>[3x]SGFVCNTCPEKWINFQRKCYYFGKGTKQWVHARYACDDMEGQLVSIHSPEEQDFLTKHASHTGSWIGLRNLDLKGEFIWV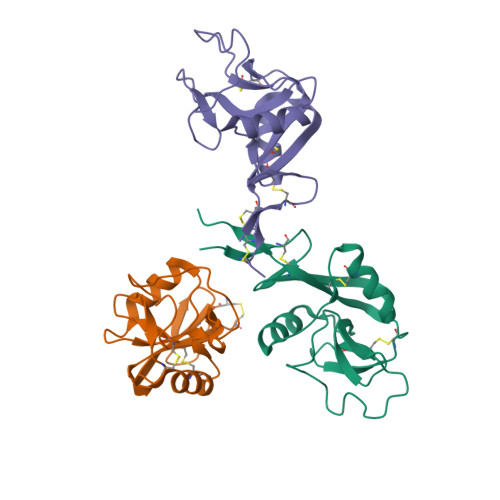DGSHVDYSNWAPGAPTSRSQGEDCVMMRGSGRWNDAFCDRKLGAWVCDRLATCTPPASEGSAE>[8x]GSSHHHHHHSSGLVPGGSHMVSKGEENNMAVIKPDMKIKLRMEGAVNGHPFAIEGVGLGKPFEGKQSMDLKVKEGGPLPFAYDILTTVFCYGNRVFAKYPENIVDYFKQSFPEGYSWERSMNYEDGGICNATNDITLDGDCYIYEIRFDGVNFPANGPVMQKRTVKWEPSTEKLYVRDGVLKGDVNEALSLEGGGHYRCDFKTTYKAKKVVQLPDYHFVDHHIE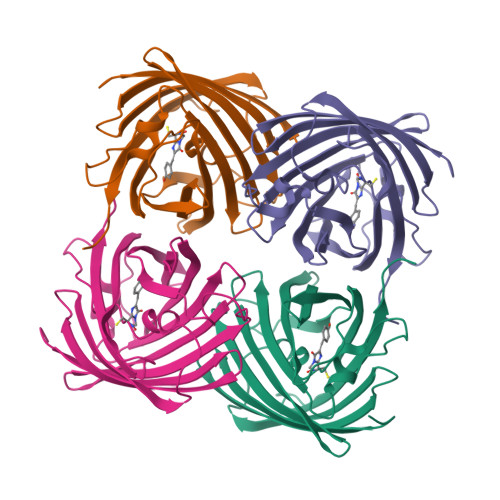IKSHDKDYSNVNLHEHAEAHSGLPRQAMDELYK> MAFDGTWKVDRNENYEKFMEKMGINVVKRKLGAH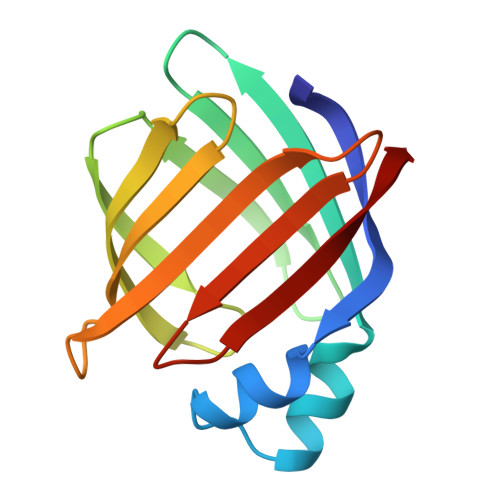DNLKLTITQEGNKFTVKESSNFRNIDVVFELGVDFAYSLADGTELTGTWTMEGNKLVGKFKRVDNGKELIAVREISGNELIQTYTYEGVEAKRIFKKE>[2x]MQDNMMWWRGGVIYQIYPRSFLDSRGDGVGDLNGITEKLDYVASLNVDGIWLSPFFTSPMLDFGYDVSDYRDVDPMFGTLEDFKALLEKAHSLGLKVMIDQVISHTSDQHPWFQESRQNRTNPKADWFVWADPKPDGTPPNNWLSIFGGSAWTFDSRRQQYYLHNFLTSQPD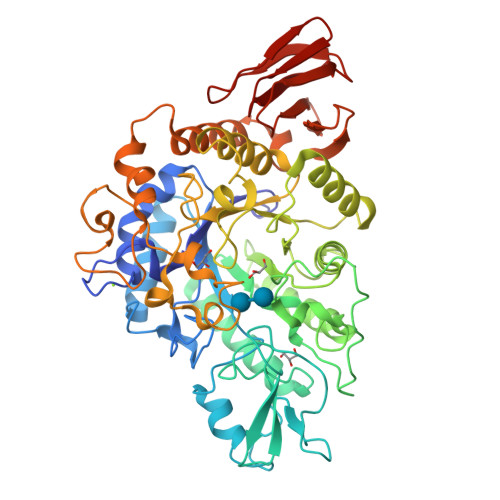VNFHHPEARQAQLDNMRFWLDLGVDGFRLDTVNFYFHDAELRDNPPVPKGEAKTLGAPEANPYTWQRHVYDLSRPENLDFLKDLRALMDEYPGTTTVGQIGDDNPLERMAEYTAGGDKLHMAYTFDLLNMPHSASYLREVIERFQRLAGDAWPCWATSNHDVVRSATRWGADEDPHAYPKVMLAVLFSLRGSVCLYQGEELGLPEADVPFERIQDPYGKVLWPEFKGRDGCRTPMPWTDGEQGGFSPVEPWLPMEARHLELAVSRQQDDPNATLNTVRALLAFRRSHPALFDGDLSLVDVGDDLLGFTRQKGDETLLCVFNLTGQEQQTTLPVEVASDLPVAHFTATRDGSTLTLPAYQAAFMQVA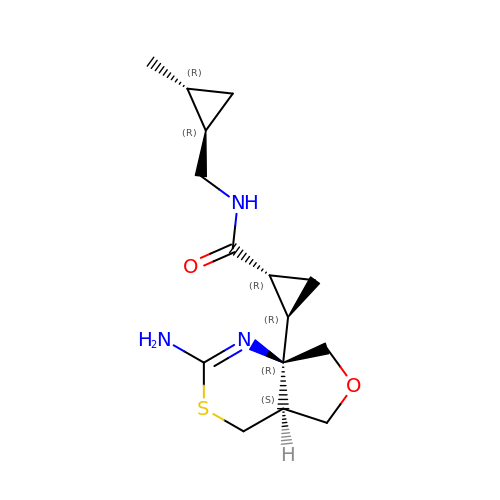(1R,2R)-2-[(4aS,7aR)-2-amino-4a,5-dihydro-4H-furo[3,4-d][1,3]thiazin-7a(7H)-yl]-N-{[(1R,2R)-2-methylcyclopropyl]methyl}cyclopropane-1-carboxamide | C15 H23 N3 O2 S | FKPBYKKZZCOMKI-MIDHOLSSSA-N>[4x]GPMEEQREILEQSKKTLQMLTVEPSKNNQIANEEKEKKENENSWCILEHNYEDIAQEFIDFIYKNPTTYHVVSFFAELLDKHNFKYLSEKSNWQDSIGEDGGKFYTIRNGTNLSAFILGKNWRAEKGVGVIGSHVDALTVKLKPVSFKDTAEGYGRIAVAPYGGTLNELWLDRDLGIGGRLLYKKKGTNEIKSALVDSTPLPVCRIPSLAPHFGKPAEGPFDKEDQTIPVIGFPTPDEEGNEPPTDDEKKSPLFGKHCIHLLRYVAKLAGVEVSELIQMDLDLFDVQKGTIGGIGKHFLFAPRLDDRLCSFAAMIALICYAKDVNTEESDLFSTVTLYDNEEIGSLTRQGAKGGLLESVVERSSSAFTKKPVDLHTVWANSIILSADVNHLY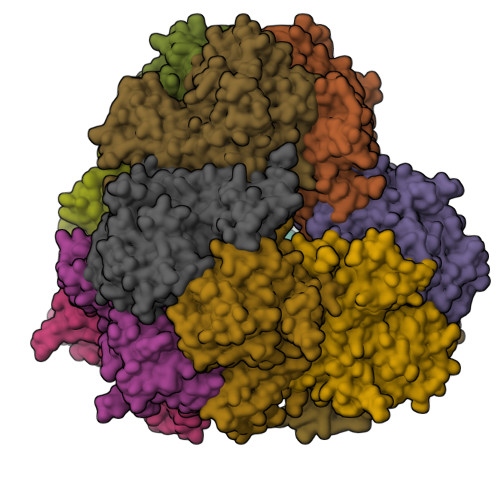NPNFPEVYLKNHFPVPNVGITLSLDPNGHMATDVVGTALVEELARRNGDKVQYFQIKNNSRSGGTIGPSLASQTGARTIDLGIAQLSMHSIRAATGSKDVGLGVKFFNGFFKHWRSVYDEFGEL> MNVLIIGKGGREHTLAWKAAQSSLVENVFAAPGNDGMAASAQLVNIEESDHAGLVSFAKQNQVGLTIVGPEVPLIEGLVDE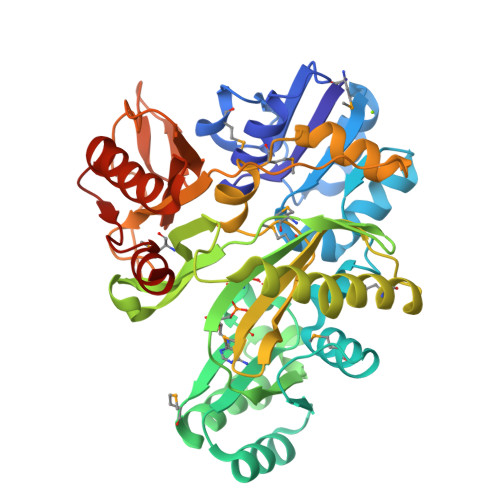FEKAGLHVFGPSKAAAIIEGSKQFAKDLMKKYDIPTAEYETFTSFDEAKAYVQEKGAPIVIKADGLAAGKGVTVAMTEEEAIACLHDFLEDEKFGDASASVVIEEYLSGEEFSLMAFVKGEKVYPMVIAQDHKRAFDGDKGPNTGGMGAYSPVPQISEETVRHAVETIVKPAAKAMVQEGRSFTGVLYAGLMLTENGSKVIEFNARFGDPETQVVLPRMESDLVQVLLDLLDDKEVDLRWKDTAAVSVVLASEGYPESYAKGTPIGSLAAETEQVVVFHAGTKAEGGEFVTNGGRVANVTAFDETFEAARDRVYKAVDEIFKPGLFFRKDIGARALKAAQK>EIQEAYILSGARTPTAKFNGSFVSVSAPELGAVAIKSAVSKSGVPVEKITDVYMGNVLQGAVGQAPARQASMFAGLSPTVESMTVNKVCASGLKAVALAAQNIQLGL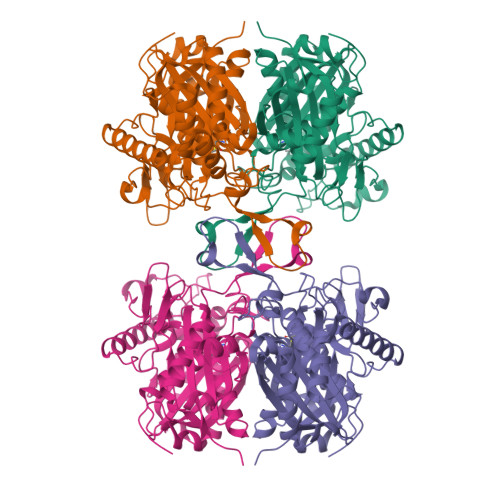AEAQVAGGMENMSRVPYYLPRSTQLPPFGEIKLQDGLIQDGLWDVYNQFHMGICAEKTAKKYEISREEQDQYAIQSYQRAQAAWKENKFAEEIAPVTVKGKKGETVVERDEGYENLRIDKMATLKPAFLRDGTGTVTAGNASTMNDGASALVLGSKAIAREFAQGNRALARIVSTADAAIDPVDFPVAPAKAVPIALERAGITKDQVAVWEFNEAFAAVIKANEKILGLQNARVNPLGGAISLGHALGSSGSRILVTLLHQLQPGEYGVAAICNGGGAATAMVVQKLDRV[4x]> MATLTAKNLAKAYKGRRVVEDVSLTVNSGEIVGLLGPNGAGKTTTFYMVVGIVPRDAGNIIIDDDDISLLPLHARARRGIGYLPQEASIFRRLSVYDNLMAVLQIRDDLSAEQREDRANELMEEFHIEHLRDSMGQSLSGGERRRVEIARALAANPKFILLDEPFAGVDPISVIDIKRIIEHLRDSGLGVLITDHNVRETL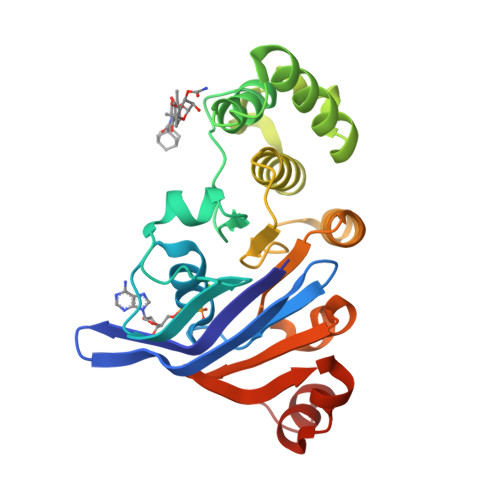AVCERAYIVSQGHLIAHGTPTEILQDEHVKRVYLGEDFRL> MDKKILVVDDEKPIADILEFNLRKEGYEVHCAHDGNEAVEMVEELQPDLILLDIMLPNKDGVEVCREVRKKYDMPIIMLTAKDSEIDKVIGLEIG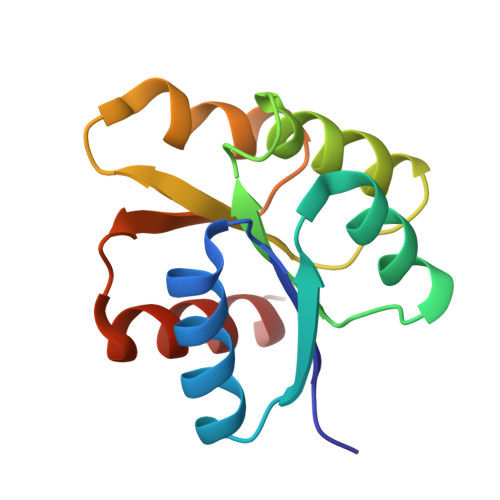ADDYVTKPFSTRELLARVKANLRRQ>[2x]MASMTGGQQMGRGSMNKPQSWEARAETYSLYGFTDMPSLHQRGTVVVTHGEGPYIVDVNGRRYLDANSGLWNMVAGFDHKGLIDAAKAQYERFPGYHAFFGRMSDQTVMLSEKLVEVSPFDS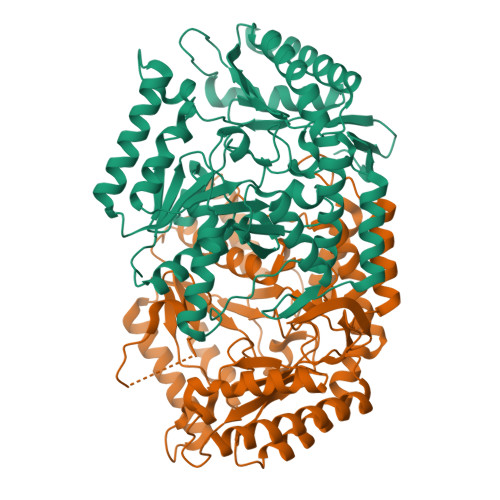GRVFYTNSGSEANDTMVKMLWFLHAAEGKPQKRKILTRWNAYHGVTAVSASMTGKPYNSVFGLPLPGFVHLTCPHYWRYGEEGETEEQFVARLARELEETIQREGADTIAGFFAEPVMGAGGVIPPAKGYFQAILPILRKYDIPVISDEVICGFGRTGNTWGCVTYDFTPDAIISSKNLTAGFFPMGAVILGPELSKRLETAIEAIEEFPHGFTASGHPVGCAIALKAIDVVMNEGLAENVRRLAPRFEERLKHIAERPNIGEYRGIGFMWALEAVKDKASKTPFDGNLSVSERIANTCTDLGLICRPLGQSVVLCPPFILTEAQMDEMFDKLEKALDKVFAEVAAAALEHHHHHH> GAMGSSTEDASQYYCDKNDNGDSYLVLIRITPDEDGKFGFNLKGGVDQKMPLVVSRINPESPADTCIPKLNEGDQIVLINGRDISEHTHDQVVMFIKASRESHSRELALVIRRR;> RQNRVDSKETEC

PTPN3 is a multidomain protein of 913 amino acids comprising a N-terminal FERM domain that determines subcellular localization, a central PDZ domain involved in protein-protein interactions, a short linker of 30-residues and a C-terminal protein tyrosine phosphatase (PTP) domain able to dephosphorylate protein substrates. The human protein tyrosine phosphatase non-receptor type 3 (PTPN3) is a phosphatase containing a PDZ (PSD-95/Dlg/ZO-1) domain that has been found to play both tumor-suppressive and tumor-promoting roles in various cancers, despite limited knowledge of its cellular partners and signaling functions. We solved the crystal structures of the complexes formed by PTPN3-PDZ with peptides comprising the PBMs of HPV 18 E6 (PBM-18E6) and of the cellular partner TACE (PBM-TACE). In all cases, the overall PDZ fold of PTPN3-PDZ is highly conserved, and the peptides bind in the conventional mode as an anti-parallel extension to the β2-strand.

PTPN3 also regulates the activity and expression of the Tumor necrosis factor alpha-convertase (TACE) protein, which impacts the release of soluble tumor necrosis factor α (TNF-α). In that case, PTPN3 was reported to bind TACE through a PDZ-PBM interaction. We determined the dissociation constant (KD) of PTPN3-PDZ for the PBM-TACE peptide comprising the last C-terminal 12-residues of TACE and encompassing the PBM (sequence RQNRVDSKETEC) following the 1H, 15N chemical shift perturbations of PTPN3-PDZ NMR signals in the 1H-15N HSQC spectra as a function of peptide concentration. The PBM-TACE peptide binds to PTPN3-PDZ with a KD value of 30 μM. An interesting feature of PBM-TACE and PBM-HBc is the presence of the C-terminal cysteine at P0. We observed that in the complexes of PTPN3-PDZ with PBM-TACE and PBM-HBc, the cysteine side chain is oriented towards the interior of the peptide-binding groove, without making any contacts with the hydrophobic side chains that line this pocket. The cysteine side chain is short enough to fit within the binding pocket and occupies the same position as the conventional leucine side chain at P0 of HPV16 E6. At P-1, the Q side chain of PBM-16E6 and PBM-HBc and the E side chain of PBM-TACE form a H-bond with a water molecule that is in turn bonded to the Nδ2 of N524 in the β2-strand of PTPN3-PDZ. Lastly, the side chain of K526 from the β2-strand is pointed towards PBM-HBc and PBM-TACE, allowing its Nζ to form H-bonds with the carbonyl oxygen of the K or R at P-4 and with the side chain hydroxyl of S at P-5, contributing to the stability of the complex. Forming a H-bond with the short, polar side chain of S could favor the K526 side chain to orient towards the peptide, while in the other cases it adopts an extended conformation to maximize the hydrophobic contacts with the Cβ-Cγ carbon chain of E at P-3.>CPRFLKVKNWETDVVLTDTLHLKSTLETGCTEHICMGSIVLPSQHTRKPEDVRTKDQLFPLAKEFLDQYYSSIKRFGSKAH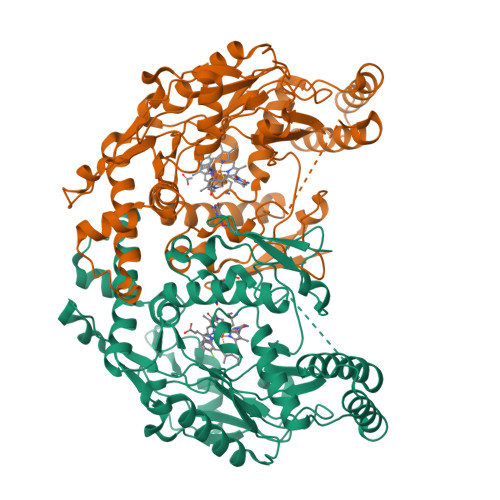MDRLEEVNKEIESTSTYQLKDTELIYGAKHAWRNASRCVGRIQWSKLQVFDARDCTTAHGMFNYICNHVKYATNKGNLRSAITIFPQRTDGKHDFRVWNSQLIRYAGYKQPDGSTLGDPANVQFTEICIQQGWKAPRGRFDVLPLLLQANGNDPELFQIPPELVLEVPIRHPKFDWFKDLGLKWYGLPAVSNMLLEIGGLEFSACPFSGWYMGTEIGVRNYCDNSRYNILEEVAKKMDLDMRKTSSLWKDQALVEINIAVLYSFQSDKVTIVDHHSATESFIKHMENEYRCRGGCPADWVWIVPPMSGSITPVFHQEMLNYRLTPSFEAQPDPWNTHVWKG[2x]>[2x]SIAWSVDEFFKNREGTFVIQEVKEKSPWVYNKKRAKERFAPQSTFKVANALIGLQTGAVRDEYDIKYWDGVKR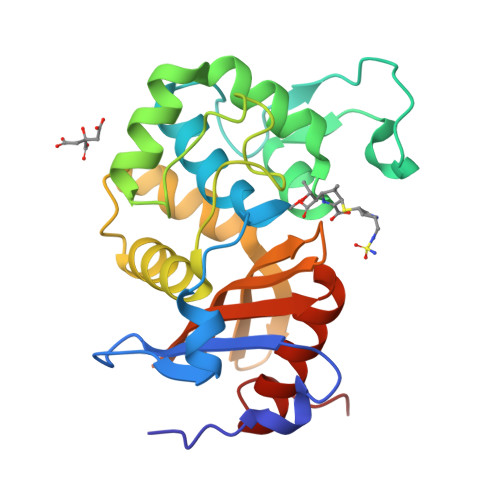EIDNWNRDHTLGSGMRDSVVWYYQAMARDIGEERMNHWVKAIHYGNKDISGGIDQFWLSSTLRISPIEQVRFLKQLYEETLPFDLKNMRTVKRMMVQEEEKHATLYGKTGSGSDIGWYVGFIKHEHKTYILATNIKGTGIEAKDITYRILKKYHLMEASV> MIGGLFIYNHKGEVLISRVYRDDIGRNAVDAFRVNVIHARQQVRSPVTNIARTSFFHVKRSNIWLAAVTKQNVNAAMVFEFLYKMCDVMAAYFGKISEENIKNNFVLIYELLDEILDFGYPQNSETGA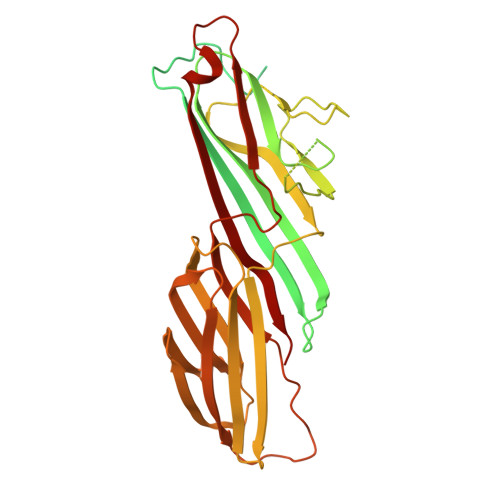LKTFITQQGIKSQHQTKEEQSQITSQVTGQIGWRREGIKYRRNELFLDVLESVNLLMSPQGQVLSAHVSGRVVMKSYLSGMPECKFGMNDKIVIEKQGKGTADETSKSMEQKLISEEDLGKQSIAIDDCTFHQCVRLSKFDSERSISFIPPDGEFELMRYRTTKDIILPFRVIPLVREVGRTKLEVKVVIKSNFKPSLLAQKIEVRIPTPLNTSGVQVICMKGKAKYKASENAIVWKIKRMAGMKESQISAEIELLPTNDKKKWARPPISMNFEVPFAPSGLKVRYLKVFEPKLNYSDHDVIKWVRYIGRSGIYETRC>MHHHHHHLEVLFQGPLGSEFRAGMTFEYITGKTGLKEICKRLEKSPYLYLATATTGNRIRLVQLGDDEKTYVIDLYEIHDITPLRELISEKGVIGHNLKFDLHYLMNYQIEPLATFDTMIASFLLGYERHSLNHLVGNLLGYTLDKSYQLSDWGAPVLSDAQLKYAAKDVDVLRELFPKLRDMLNELEGERGEELLKTRTARIFGLKSPVAIVEMAFVKEVAKLERNGLPVDIETLESTLKDIERKTQKKVQEFLIKFRVDPFSPKQVGQLLTSKYKLNLPRTQKGNVSTDDKVLSSYAHVEPVRLLLEIRKLKKLSDKFKEIKENLKGDRLYPEFKQIGAVTGRMSSLKPNVQNVPREERAIFKAPEGNTFVIADFSQIELRIAAEYVNEELMIRAFREGKDLHRYTASLVLGKRE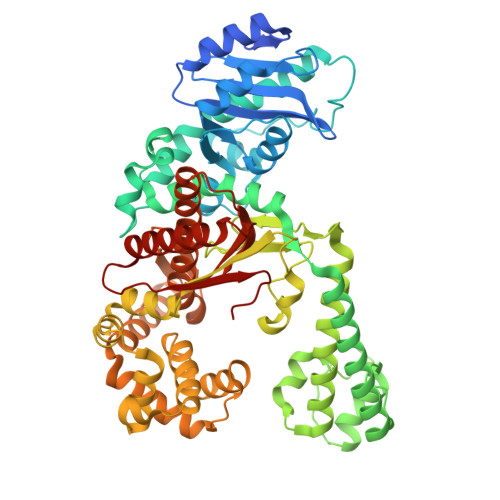EEITKEERQLAKAINFGLIYGISAKGLAEYARTGYGVEISEEEAETFRNRFFKNFKAFKLWHEKVKKELKEKGVFRGRTLLGRRFTATTFNDAVNYPIQGTGADLLKLAVLLFDAEAKKKKLDAKLVNLVHDEIVVECRKEVANQVKEVLEKAMKQAGKIILKKVPVEVESVINERWIKD[2x]N~2~-({3-HYDROXY-2-METHYL-5-[(PHOSPHONOOXY)METHYL]PYRIDIN-4-YL}METHYL)-L-LYSINE | C14 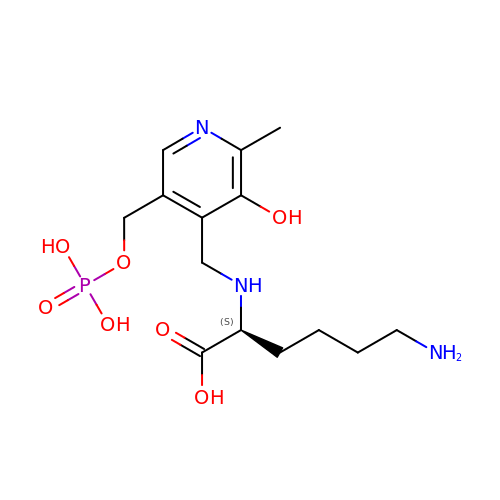H24 N3 O7 P | GQMAOPRRHWJXFB-LBPRGKRZSA-N> TTWKEATLPQVKAMLEKDDGKVSGDT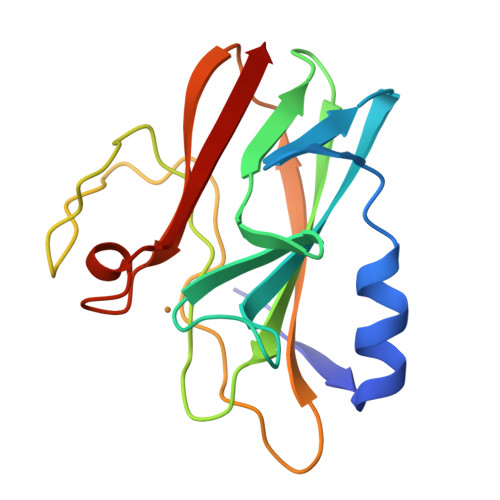VTYSGKTVHVVAAAVLPGFPFPSFEVHDKKNPTLEIPAGATVDVTFINTNKGFGHSFDITKKGPPYAVMPVIDPIVAGTGFSPVPKDGKFGYTDFTWHPTAGTYYYVCQIPGHAATGMFGKIVVK>METDNVELAQSKRKVVLAEQGSFYIGGRTVTGPGKFDPSKPVIRYSNEGATFYINQMYVNFQAPVRPRGLPLVFWHGGGLTGHIWESTPDGRPGFQTLFVQDRHTVYTIDQPGRGRGNIPTFNGPFGQLEEESIVNTVTGNSSKEGAWVRDRLGPAPGQFFENSQFPRGYEDNYFKEMGFSPSISSDEIVDAVVKLVTHIGPCVLVTHAASGVLGMRVATHAKNVRGIVAYEPATSIFPKGKVPEIPPLADKKSQIFPPFEIQESYFKKLAKIPIQFVFGDNIPKNPKSAYWFLDWWRVTRYAHSLSLEAINKLGGQASLLD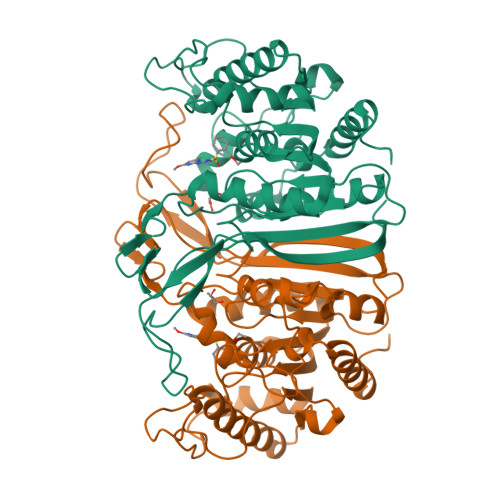LPTAGLRGNTAFPFTDRNNVQVASLLSDFLGKHGLDQNESLEHHHHHH[2x]N-1H-indazol-5-yl-2-(6-methylpyridin-2-yl)quinazolin-4-amine 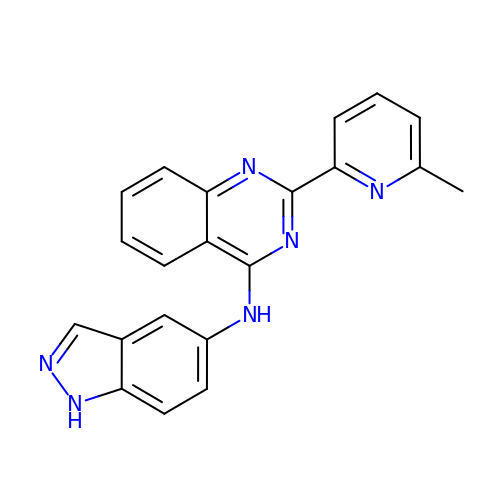| C21 H16 N6 | HNHRWNUXTCATSG-UHFFFAOYSA-N INOSITOL-2-METHYLENE-1,2-CYCLIC-MONOPHOSPHATE 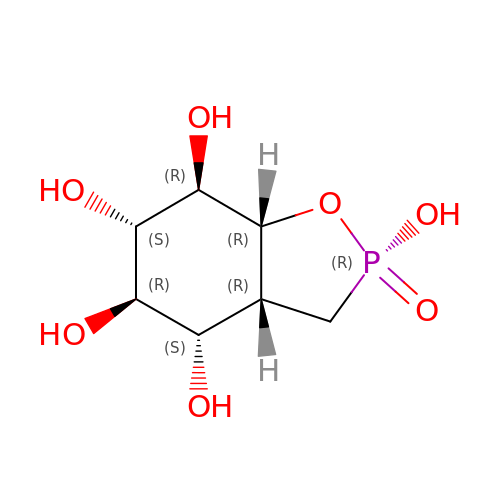| C7 H13 O7 P | HSPMBPCIFXNUBY-YXVPSNDASA-N>SNAVGRLEGKIAIVTGAASGIGAVTAERLAAEGARVALADLDAVGVQTLAEKIRGADGTHAIGIEVDLADPASVRAMVAAAVEEFGGLDILHNNAAATALASSLDVPVADADPEVWDRTMRVNLSGAMVATQAALPHLIARGGGCVINTSSAAGLSGDLSHPAYAASKAALISLTRSVATQAGRSGVRCNAIAPGLIITRPEREAAYRVMLPHHLTTRLGRPEDVASAVVFLASDEASFITGQTLVVDGGLLAHQPYYADRRA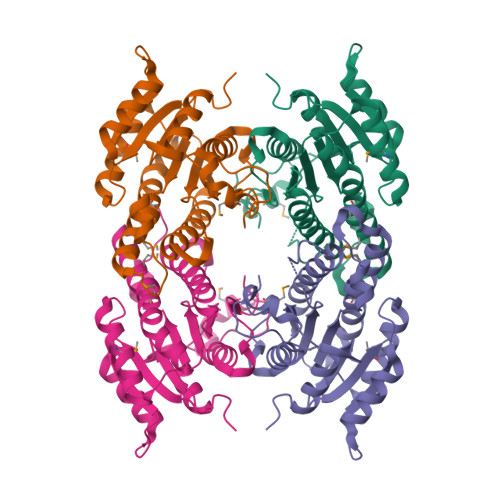ET[2x]> MTDVARLLALRSFTELGARQRARALLDAGSFRELLDPFAGVQSPWLERQGIVPQADDGVVVARGLLDGQPAVLAAIEGAFQGGSLGEVSGAKIAGALELAAEDNRNGVPTRALLLLETGGVRLQEANLGLAAIAEIQAAIVDLQRYQPVVAVIAGPVGCFGGMSIAAGLCSYVLVTREARLGLNGPQVIEQEAGIAEYDSRDRPFIWSLTGGEQRFASGLADAYLADDLDEVRTSVLAYFAKGLPARPRCRRAEDYLRRLGDLDTAEQPDAAGVRRLYQGLGQG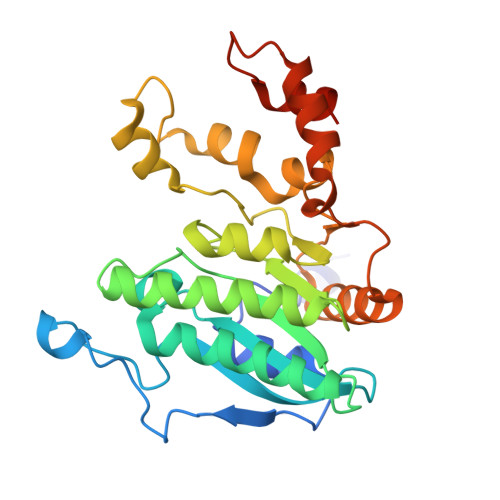DAT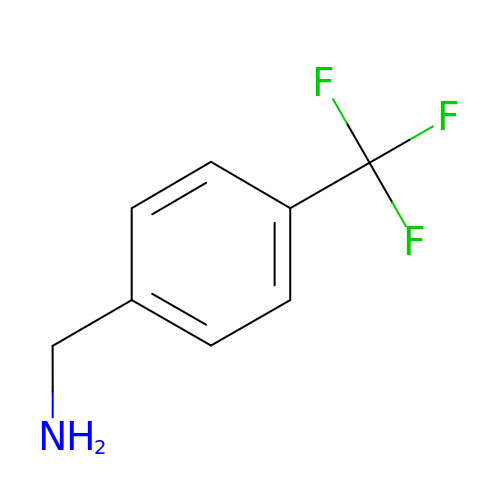[4-(trifluoromethyl)phenyl]methanamine | C8 H8 F3 N | PRDBLLIPPDOICK-UHFFFAOYSA-N>[2x]MSDSQTLVVKLGTSVLTGGSRRLNRAHIVELVRQCAQLHAAGHRIVIVTSGAIAAGREHLGYPELPATIASKQLLAAVGQSRLIQLWEQLFSIYGIHVGQMLLTRADMEDRERFLNARDTLRALLDNNVVPVINENDAVATAEIKVGDNDNLSALAAILAGADKLLLLTDQKGLYTADPRSNPQAELIKDVYGIDDALRAIAGDSVSGLGTGGMS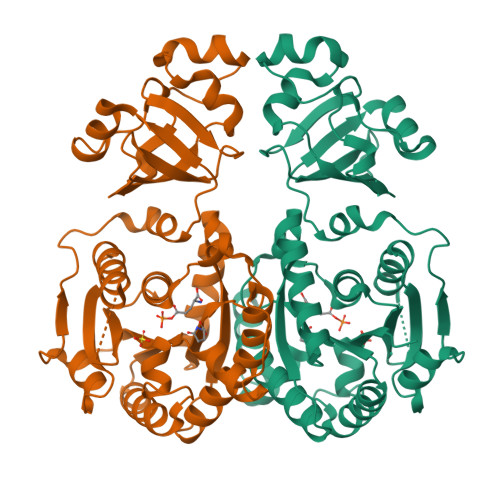TKLQAADVACRAGIDTIIAAGSKPGVIGDVMEGISVGTLFHAQATPLENRKRWIFGAPPAGEITVDEGATAAILERGSSLLPKGIKSVTGNFSRGEVIRICNLEGRDIAHGVSRYNSDALRRIAGHHSQEIDAILGYEYGPVAVHRDDMITR>[2x]METDAFYKREMFDPAEKYKMDHRRRGIALIFNHERFFWHLTLPERRGTCADRDNLTRRFSDLGFEVKCFNDLKAEELLLKIHEVSTVSHADADCFVCVFLSHGEGNHIYAYDAKIEIQTLTGLFKGDKCHSLVGKPKIFIIQACRGNQHDVPVIPL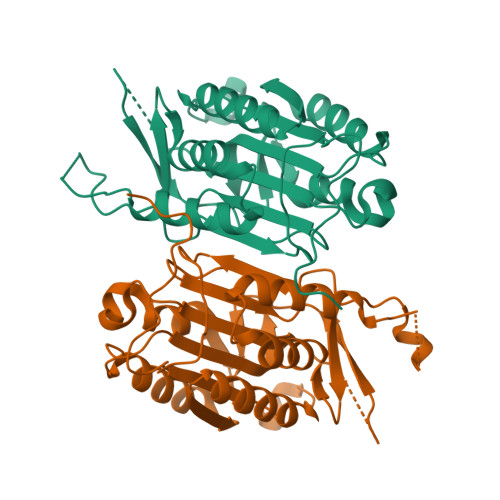DVVDNQTEKLDTNITEVDAASVYTLPAGADFLMCYSVAEGYYSHRETVNGSWYIQDLCEMLGKYGSSLEFTELLTLVNRKVEQRRVDFCKDPSAIGKKQVPCFASMLTKKLHFFPKSNLEHHHHHH> SEDKRAKVTSAMQTMLFTMLRKLDNDALNNIINNARDGCVPLNIIPLTTAAKLMVVIPDYNTYKNTCDGTTFTYASALWEIQQVVDA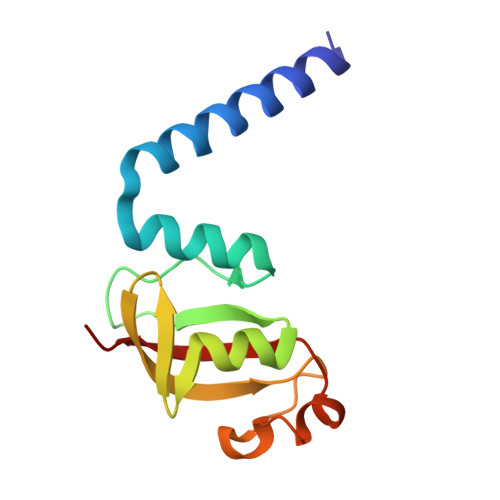DSKIVQLSEISMDNSPNLAWPLIVTALRAN>[2x]MSFVLFLSFLLFVSAVTCFSTNWRSDEEVIALYEEWLAKHQKLHSSLRENIEIEIFKDNLRYIDEQNNYNKFNHKNFTLGLNQFADLTLDEFSSIYLGTSIEYDPIISSNPNHHGEEEDILQEGAIELPNSVDW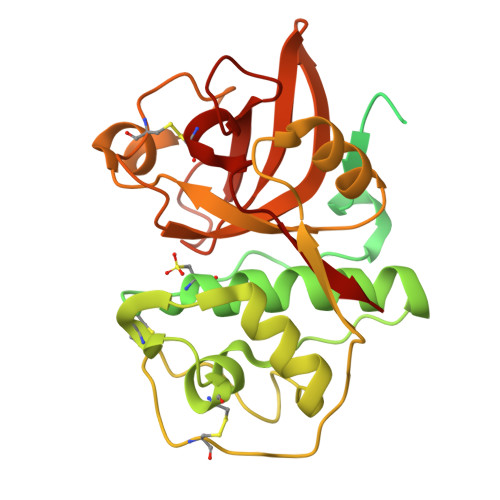REKDVVFPIRNQGQCGSCWTFSAVASIETLIGIKEDRMIALSEQELLDCERTSYGCKGGYYTDAFAYVAKKGLTSREKYPYIFQQGQCYQKEKVVKISGYRRIPKNDEKKLQSVVAQQVVSVGVKSKSRDFQHYRSGVFSGACGPRVDHAVNIVGYGSEGGVNYWIVRNSWGTNWGENGYMRIPRNSNQSGGYCGIAVQAAYPVY> PGSMTLSSNQYQLPLNVRPYTTTWCSQSPSCSNLLAIGHDTGITIYCASEEQTPGSTGLTLQELFTIQTGLPTLHLSFSSSCSYSENLHDGDGNVNSSPVYSLFLACVCQDNTVRLIITKNETIITQHVLGGKSGHHNFVNDIDIADVYSADNRLAEQVIASVGDDCTLIIWRLTDEGPILAGYPLSSPGISVQFRPSNPNQLIVGERNGNIRIFDWTLNLSAEENSQTELVKNPWLLTLNTLPLVNTCHSSGIASSLANVRWIGSDGSGILAMCKSGAWLRWNLFANNDYNEISDSTMKLGPKNLLPNVQGISLFPSLLGACPHPRYMDYFATAHSQHGLIQLINTYEKDSNSIPIQLGMPIVDFCWHQDGSHLAIATEGSVLLTRLMGFTRL;> PGSMNELKHAVVPIDLQSFCLEGTLALWVPALENDSEDDSEAIETADDNEKLFKKECVAYDAGVYTSNKSKGSQTLRWSIFQNRTLTIFDVSLNSKKEPLSKFNVKIHFPSNVMKDGVAFSFSEHSDTTIIYAITHARVLYYIRLSKTWFQLPDARLDDDWCLCYRPISFLNQKPDLMAAISTSEICVSFFNGGLTKIILNPKDASHYEQHIDDSSYLFSLKKYLSLQAFKADYRSPNTIISMIFLSTYNVLVMLSLDYKLKVLDLSTNQCVETIELSQTILPLQSFPYLTSDHTTNSFIALYYPDNSHGSFSIYKLNANAHSFKLNVVIEKGIIPPSLPDDEFIPWMLSDFQLISSEGSQSKFLLIIAWKSNLNTVIQKCNLSLDQDESFSCVWSHSLDSFSLIEKTFFDVPTNMSSGDISEIWLQHIFAHNTSIESIQVALLSFQNSSSQVSKNKLDKFGALTISELKNAVLSSIVSTIQIEPNSDLTGYDYYEYKRLLYNEWERFAKLVAYLDHFGDEILSINFDPSNAVTYINYANKVAFIRDPYLIESFDEEPLTKLISSLETDDPSLIEGYQILDLGRSLHSCMSFSTLSEIRYSLRELVQDLPSYSLFDTLWVFYDKHIYPNVD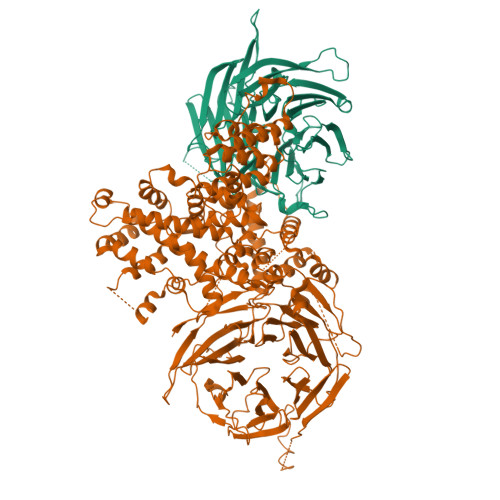PDYISTLIDTLVSLENPMRDIDSLIQRLRSFDIYNHSAQSPSLFLCASVARVLDSILKKFQVSIEGFIFLLSLITSQQDYELQSKFAGCDKLFLSLLEDWRLVSFLLENSALLLEKFEEEDVDSTNCNLNTMEALASVNTALQFFSALNYSECFSESQISPLHATVISSLSAIFIRDDTENDLVTELVEKLFLFKQYNACMQLIGWLNSDPIAVYLKALIYLKSKEAVKAVRCFKTTSLVLYSHTSQFAVLREFQEIAEKYHHQNLLSCYYLHLSKKLFEESAYIDALEFSLLADASKETDDEDLSIAITHETLKTACAAGKFDAAHVALMVL>MASMALVRPFPIVQVVGFQNSGKTTFIERIL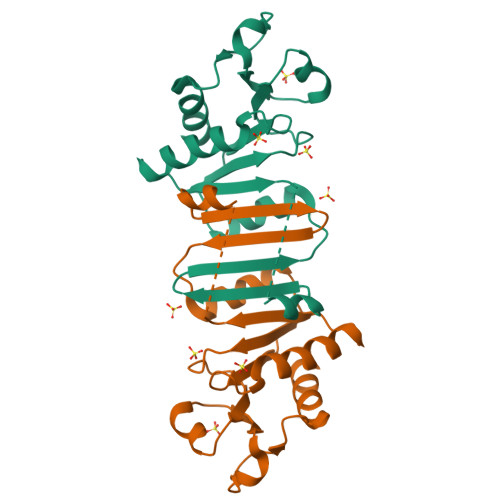EKASEQGLNLGCLKHHGHGGEPQTFTEGKDTDRYQAAGADVTAVEGAGVLQLTARRLWDLTRLIELYQFLETDCLLIEGFKKAPYPKVVILSEKEDLEALKTVNTIAIIYRKKEHMTEHQGLPIFHADDPVAVDLVLSQLKGESA[5x]> MGLFDRIKRVVSSNLNDLVNKAEDPEKMLEQAILEMQEDLVQLRQGVAQ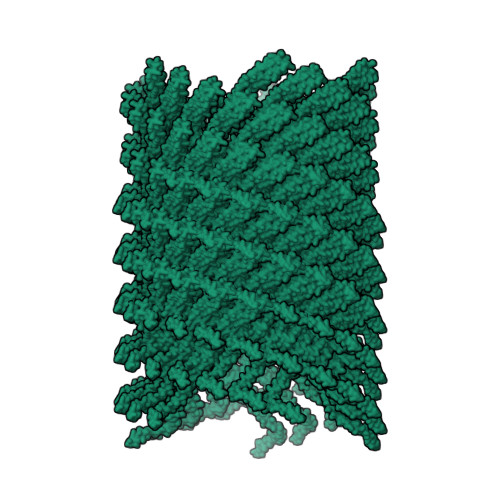AIAAQKRSEKQYNDAQNEINKWQRNAQLALQKGDENLARQALERKKTYTDTSAALKASLDTQSTQVETLKRNLIQLESKISEAKTKKEMLKARITTAKAQEQLQGMVRGMNTSSAMSAFERMEEKVLMQESRAQALGELAGADLETQFAQLEGGSDVDDELAALKAQM> TTALSLPACPEESPLL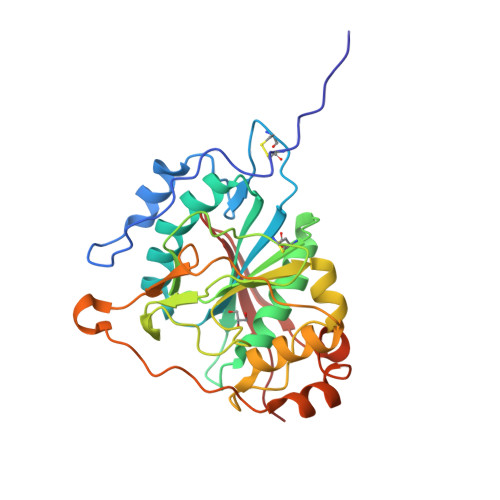VGPMLIEFNMPVDLELVAKQNPNVKMGGRYAPRDCVSPHKVAIIIPFRNRQEHLKYWLYYLHPVLQRQQLDYGIYVINQAGDTIFNRAKLLNVGFQEALKDYDYTCFVFSDVDLIPMNDHNAYRCFSQPRHISVAMDKFGFSLPYVQYFGGVSALSKQQFLTINGFPNNYWGWGGEDDDIFNRLVFRGMSISRPNAVVGRCRMIRHSRDKKNEPNPQRFDRIAHTKETMLSDGLNSLTYQVLDVQRYPLYTQITVDIGTPS> GSHMPYTIELIQPEDGEAVIAMLKTFFFKAEPLNTFLDLGECKELEKYSLKPLPDNCSYKAVNKKGEIIGVFLNGLMRRPSPDDVPEKAADSCEHPKFKKILSLMDHVEEQFNIFDVYPDEELILDGKILSV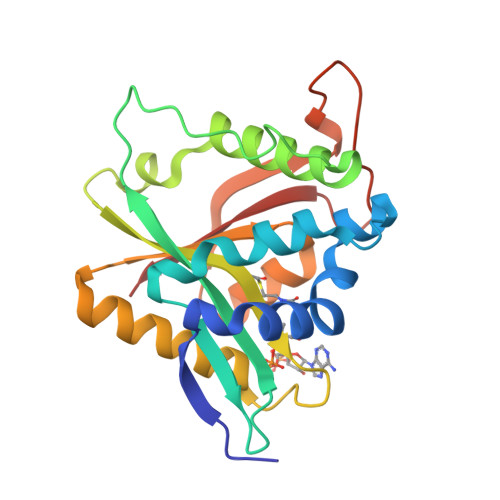DTNYRGLGIAGRLTERAYEYMRENGINVYHVLCSSHYSARVMEKLGFHEVFRMQFADYKPQGEVVFKPAAPHVGIQVMAKEV Interestingly, human SCL (hSCL) is unlike several bacterial orthologues specific for Sec and does not accept the sulfur analogue Cys as substrate with any appreciable activity. SCL and CD enzymes are NifS-like proteins that contain a completely conserved active site Cys residue (C388, hSCL numbering) that form an enzyme-bound persulfide (Cys-S-SH) or sulfoselenide (Cys-S-Se−) as product of the reactions with Cys or Sec, respectively. Similar to the non-specific SCL/CD enzymes, hSCL was found to adopt the canonical fold type I structure of PLP enzymes, forming two active sites in the homodimer interface with each monomer contributing residues to both active sites. Structures of hSCL in two different crystal forms were determined: P1 to 1.8 Å, with four monomers per asymmetric unit and P212121 to 2.1 Å resolution, with two monomers per asymmetric unit.

In the P212121 structure, the segment containing C388 (residues 385–396) was ordered in both subunits of the asymmetric unit. Interestingly, it adopted two different ordered conformations in the two monomers. In subunit A, the segment was folded onto the protein in a near α-helical “closed” conformation, restricting access to the active site and placing the active site C388 in proximity to the PLP cofactor. In contrast, the corresponding active site segment of subunit B displayed an extended β-hairpin structure, positioning C388 more than 17 Å from the PLP cofactor and exposing it to solvent. Remarkably, in spite of the completely different backbone architecture, the closed conformation of hSCL positioned the C388 sulfur atom in an identical position in relation to the PLP cofactor and substrate-binding site as observed in the group-II proteins. The persulfide adduct was present in subunit A with near full occupancy and also in subunit D, but there at lower occupancy. Together, this strongly suggests that the closed conformation observed in the present structure is involved in catalysis and C388-sulfoselenide formation using Sec as a substrate. It should be noted that although the dynamic segment (residues 385–396) was visible in the electron density in both subunits in the P212121 structure it seemed less rigid than the rest of the protein, as indicated by higher B-factors and a somewhat weaker electron density. In particular the density for Gly 393 of subunit B was poor. The hSCL structure shows that in the closed state, relevant for sulfoselenide formation, the reactive sulfur atom of C388 is buried in the protein and completely covered by the residues of the dynamic segment. However, in the open form, the sulfur atom is exposed and accessible to solvent.

>SMGRDAPAPAASQPSGCGKHNSPERKVYMDYNATTPLEPEVIQAMTKAMWEAWGNPSSPYSAGRKAKDIINAARESLAKMIGGKPQDIIFTSGGTESNNLVIHSVVKHFHANQTSKGHTGGHHSPVKGAKPHFITSSVEHDSIRLPLEHLVEEQVAAVTFVPVSKVSGQTEVDDILAAVRPTTRLVTIMLANNETGIVMPVPEISQRIKALNQERVAAGLPPILVHTDAAQALGKQRVDVEDLGVDFLTIVGHKFYGPRIGALYIRGLGEFTPLYPMLFGGGQERNFRPGTENTPMIAGLGKAAELVTQNCEAYEAHMRDVRDYLEERLEAEFGQKRIHLNSQFPGTQRLPNTCNFSIRGPRLQGHVVLAQCRVLMASVGAACHSDHGDQPSPVLLSYGVPFDVARNALRLSVGRSTTRAEVDLVVQDLKQAVAQLEDQA[2x]> TESDMRATL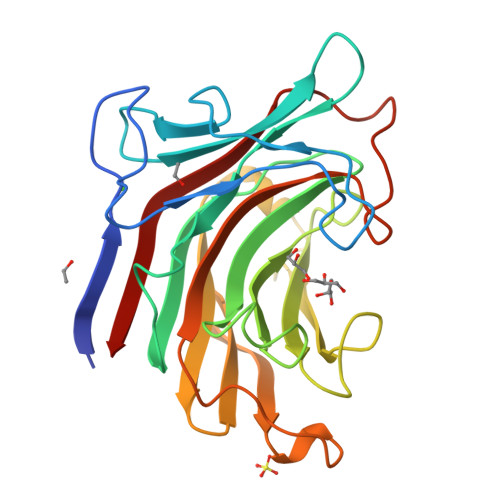VWSDEFDGPAGSAPDPANWNHETGDHGWGNNELQNYTDSRANSALDGNGNLVITARQEADGGYTSARLTTQNKVQPQYGRVEASIQIPRGQGIWPAFWMLGADFPNTPWPDSGEIDIMENIGREPHLVHGSLHGPGYFGGEPLTGSYMHPQGWSFADTFHTFAVDWRPGSITWSVDGVAYQTYTSADTRGNPWVFDQPFFMILNVAVGGDWPGYPDGSTQFPQEMRVDYVRVYELG>[2x]GSHMQVLSY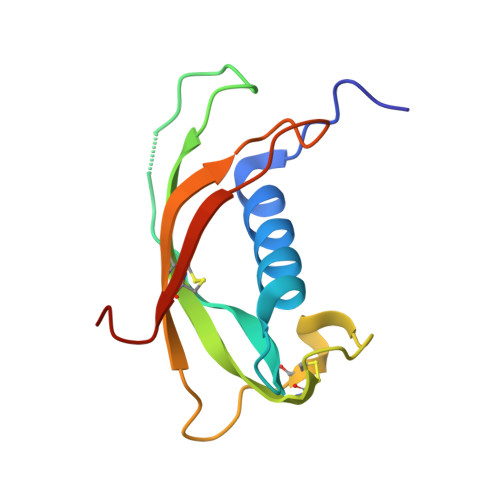KEAVLRAIDGINQRSSDANLYRLLDLDPRPTMDGDPDTPKPVSFTVKETVCPRTTQQSPEDCDFKKDGLVKRCMGTVTLNQARGSFDISCDKDNKRFA>ATQGVFTLPANTRFGVTAFANSSGTQTVNVLVNNETAATFSGQSTNNAVIGTQVLNSGSSGKVQVQVSVNGRPSD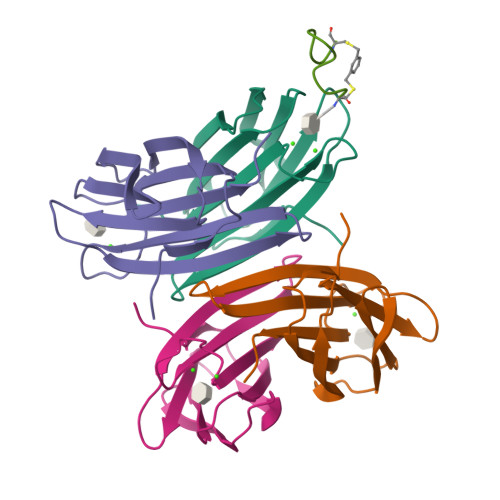LVSAQVILTNELNFALVGSEDGTDNDYNDAVVVINWPLG[4x];> CWWKKKKKWWC> GGAHKVRAGGPGLERAEAGVPAEFSIWTREAGAGGLAIAVEGPSKAEISFEDRKDGSCGVAYVVQEPGDYEVSVK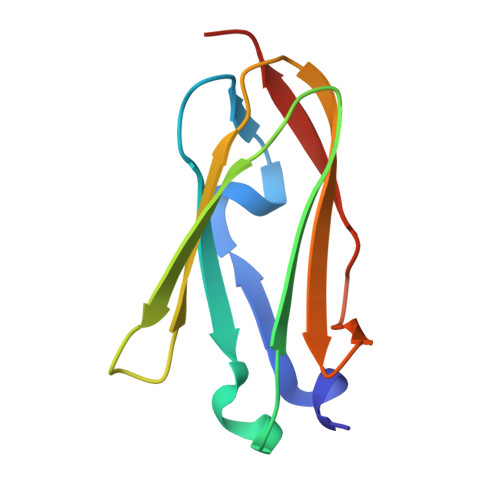FNEEHIPDSPFVVPVASPS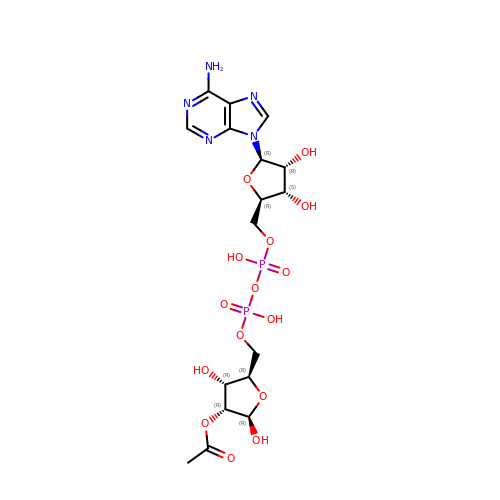[(2R,3R,4R,5R)-5-[[[[(2R,3S,4R,5R)-5-(6-aminopurin-9-yl)-3,4-bis(oxidanyl)oxolan-2-yl]methoxy-oxidanyl-phosphoryl]oxy-oxidanyl-phosphoryl]oxymethyl]-2,4-bis(oxidanyl)oxolan-3-yl] ethanoate | C17 H25 N5 O15 P2 | BFNOPXRXIQJDHO-QJWJOKBXSA-N>[2x]GAMNWTVDIPIDQLPSLPPLPTDLRTRLDAALAKPAAQQPTWPADQALAMRTVLESVPPVTVPSEIVRLQEQLAQVAKGEAFLLQGGDCAETFMDNTEPHIRGNVRALLQMAVVLTYGASMPVVKVARIAGQYAKPRSADIDALGLRSYRGDMINGFAPDA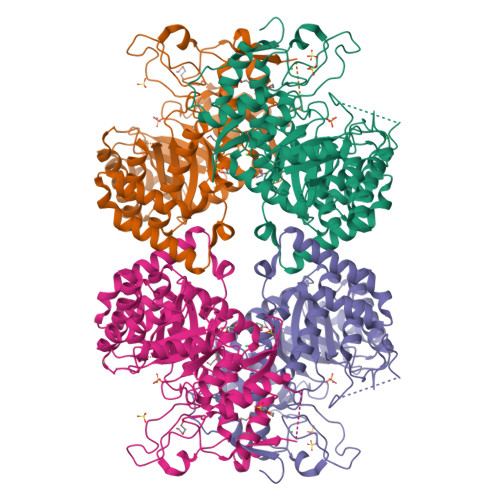AAREHDPSRLVRAYANASAAMNLVRALTSSPLASLHLVHDWNREFVRTSPAGARYEALATEIDRGLRFMSACGVADRNLQTAEIYASHEALVLDYERAMLRLSDGDDGEPQLFDLSAHTVWIGERTRQIDGAHIAFAQVIANPVGVKLGPNMTPELAVEYVERLDPHNKPGRLTLVSRMGNHKVRDLLPPIVEKVQATGHQVIWQCDPMHGNTHESSTGFKTRHFDRIVDEVQGFFEVHRALGTHPGGIHVEITGENVTECLGGAQDISETDLAGRYETACDPRLNTQQSLELAFLVAEMLRD> SMRKFSLNELAKVTSNFNAENKLGEGGFGSVYRGFLRDSDTYIAVKKVSRASKQGIKEYASEVKIISRLRHKNLVKLIGWCHERGELMLVYEFMANGSLDSHIFKGKSLLTWEVRYRIVKDLASALLYLHEEGDHCVLHRDIKTSNIMLDSSFNAKLGDFGLARLVDHAKGLKKTLLAGTVGYM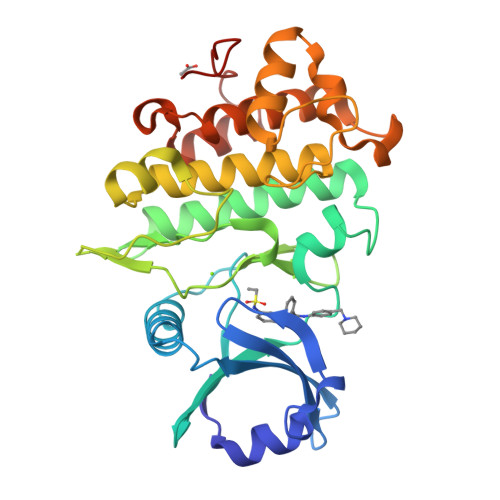APECLSSGKASKESDVYSFGVVALEIASGRRSIEPKFEESEALLLVPWVWESYGNERILDIADRKLGMAFDPKQLECLVMVGLWCAHPSHNLRPSIRQVIQVLNFEAPLPNLPGSMPIPNYNDVQ3,4-difluoro-N-({1-[(2R)-4-(hydroxyamino)-4-oxo-1-(quinolin-7-yl)butan-2-yl]-1H-1,2,3-triazol-4-yl}methyl)benzamide | 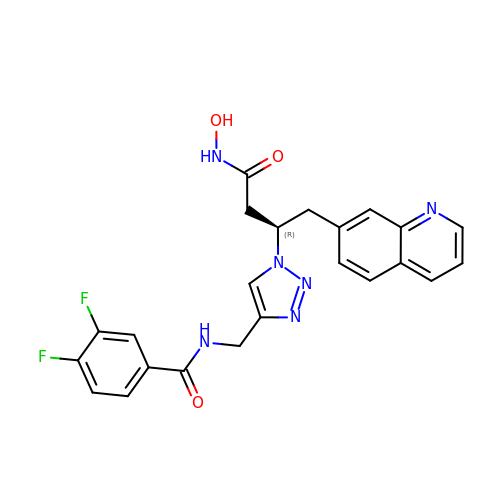C23 H20 F2 N6 O3 | NEONSMDVMOADLB-GOSISDBHSA-N> AQSVPWGISRVQAPAAHNRGLTGSGVKVAVLDTGISTHPDLNIRGGASFVPGEPSTQDGNGHGTHVAGTIAALNNSIGVLGVAPNAELYAVKVLGASGSGSVSSIAQGLEWAGNNGMHVANLSLGSPSPSATLEQAVNSATSRGVLVVAASGNSGAGSISYPARYANAMAVGATDQNNNRASFS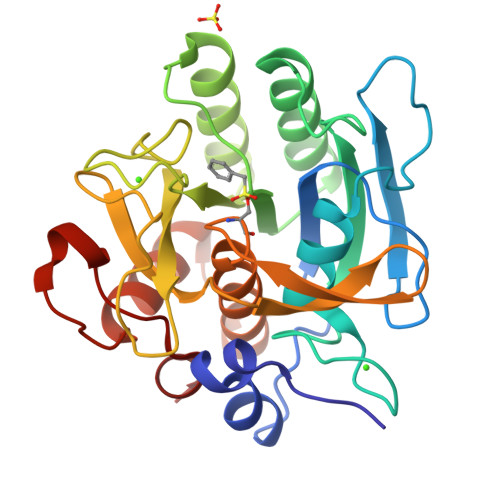QYGAGLDIVAPGVNVQSTYPGSTYASLNGTSMATPHVAGAAALVKQKNPSWSNVQIRNHLKNTATSLGSTNLYGSGLVNAEAATR> GP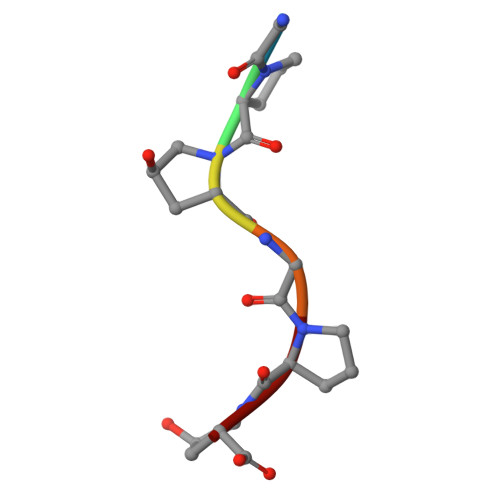PGPP beta,beta-caroten-4-one | C40 H54 O | 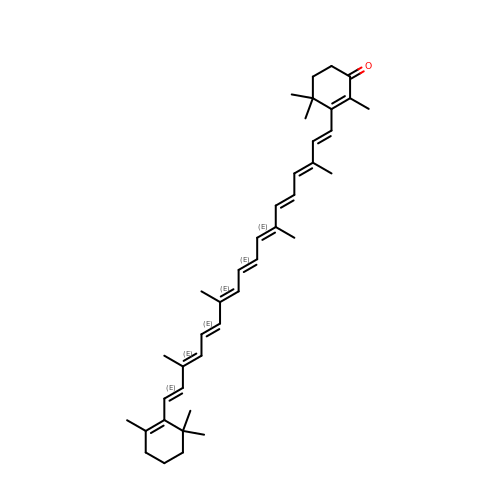QXNWZXMBUKUYMD-QQGJMDNJSA-N>MSILSLTASQGQKATALANAVATATALLAVILFAVATRAASATKAEACQTPCQCSHQLRQAAAHYNSVLREAERKTDGHILQALKLLIAATGNNQKLQAAAVAPLATALKNWANCKAETGRLGTAARNNIDKLNAGAEAAAILANLTKLGGKVELTAKGGNGQLQQDSVTAEDLWRNTATECQIEEAEQGRHNFDPANSSDKMKLPKFNPVAKIGINCKKGGDTNNCNANAMAQNTGKLQFDVKIEAMGTQGGNDAASKWESAKAAEPVYITNELNIIAKTLESAGVANQALQNEFKQNSCAEPSEEYSDFSNSGDFSRQIIRSYSNNKDNEKETTDKPSDLEKLIESAYGKNGAKFKENLWDQIDKLSPTVNKGETNEKLNLKTEKDISKLGEALARQLGYIRKEPEAAAEAQEKKTN[4x]

Long-term immune evasion by the African trypanosome is achieved through repetitive cycles of surface protein replacement with antigenically distinct versions of the dense Variant Surface Glycoprotein (VSG) coat. The mature VSG proteins are attached to the cell surface by a GPI-anchor, and consist of two main regions: (1) a large, N-terminal domain (NTD) of roughly 300–400 amino acids that is most distal to the membrane and (2) a smaller, membrane-proximal C-terminal domain (CTD) spanning 80–120 amino acids beneath the NTD that harbors the GPI-anchor. Therefore, at the heart of antigenic variation in the African trypanosome are the NTDs of the VSGs. These large subdomains are elongated folds centered on a three-helix bundle scaffold.

The structure of the VSG558 NTD was determined to 1.74 Å resolution. It has a highly similar structure to VSG13 with a 2.54 Å RMSD over 324 residues. A notable difference with all the previously solved VSG NTD structures published is the presence of two N-linked glycans at the middle lobe of the VSG558 protein. To date, all VSG structures determined have been characterized by a single N-linked glycan (or none, as seen in the case of ILTat1.24). The structure of VSG558 confirms the presence of multiple N-linked glycans for another VSG. This shows that not only are the locations of the N-linked glycans variable (found in both the bottom and middle lobes), but that the number of possible such carbohydrates is also variable. Finally, as noted in the Methods, the structures of VSG21, VSG545, VSG558, and VSG615 were solved by molecular replacement using an AlphaFold model of these VSGs as search models, indicating a very close fit of the model to the experimental data (a general idea for X-ray phasing implemented by several groups due to the accuracy of AlphaFold models).> MTVLKMTDLDLQGKRVLIREDLNVPVKDGVVTSDARILASLPTIKLALEKGAAVMVCSHLGRPTEGEFSAENSLKPVADYLSKALGREVPLVSDYLNGVDVKAGDIVLFENVRFNKGEKKNADELAKQYAALCDVFVMDAFGTAHRAEGSTHGVAKFAKVAAAGPLLAAELDALGKALGAPAKPMAAIVAGSKVSTKLDVLNSLSQICDLLIVGGGIADTFLAAAGHPVGKSLYEPDLLDTARAIAAKVNVPLPTDVVVAKEFAESAEATVKLIADVAADDMILDIGPQTAEHFAQLLKTSKTILWNGPVGVFEFDQFGNGTKVLAKAIADSAAFSIAGGGDTLAAIDKYGVADQISYISTGGGAFLEFVEGKVL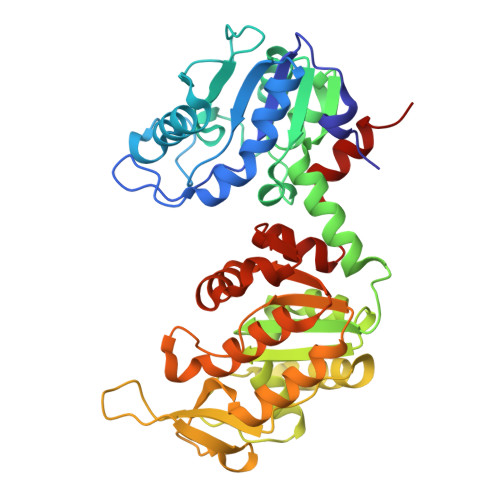PAVEVLESRAKA> SANTNHQYAVIAYFYGNASLQGANATINIWEPNLKNPNGDFSLTQIWISAGSGSSLNTIEAGWQVYPGRTGDSQPRFFIYWTADGYTSTGCYDLTCPGFVQTNNYYAIGMALQPSVYGGQQYELNESIQRDPATGNWWLYLWGTVVGYWPASIYNSITNGADTVEWGGEIYDSSGTGGFHTTTQMGSGHFP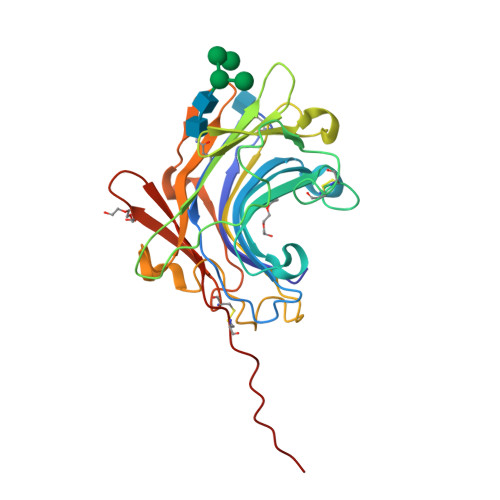TEGYGKASYVRDLQCVDTYGNVISPTANSFQGIAPAPNCYNYQFQQGSSELYLFYGGPGCQAIAHHHHHH> SGGSSARIAKAKKLIYKLEKLWNARDNDGILKLFKDDAVFNLNGVPYKGKEAIKKVLESAPKAKYKITKIDIKIV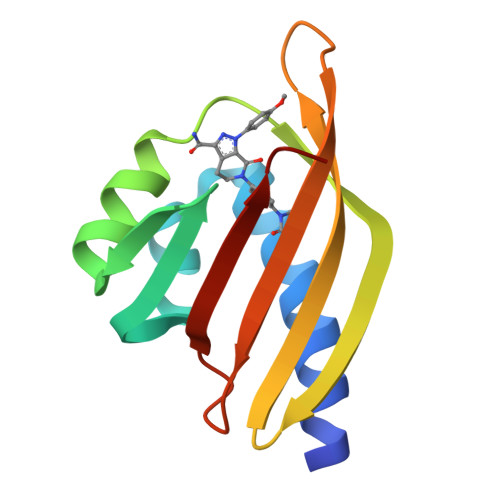GNEIIVNVDVLATGPSGFTLKVKSTITFDEDMKITSYEVNLEGS>[2x]HHHHHHSSGLVPRGSHMQETQAVEAGEKTVEQFVQALNKGDYNKAAGMASKKAANKSALSEKEILEKYQNIYGAADVKGLEISNLKVDKKDDSTYSFSYKAKMNTSLGELKDLSYKGTLDRNDGKTTINWQPNLVFPEMEGNDKVSLTTQEATRGNILDRNGEPLATTGKLKQLGVVPSKLGDGDEKTANIKAIASAFDLTEDAINQAISQSWVQPDYFVPLKIIDGATPELPAGATIQEVDGRYYPLGEAAAQLIGYVGDITAEDIDKNPELSSNGKIGRSGLEMAFDKDLRGTTGGKLSITDTDGVEKKVLIEHEVQNGKDIKLTIDAKAQKTAFDSLGGKAGSTVATTPKTGDLLALASSPSYDPNKMTNGISQEDYKAYEENPEQPFI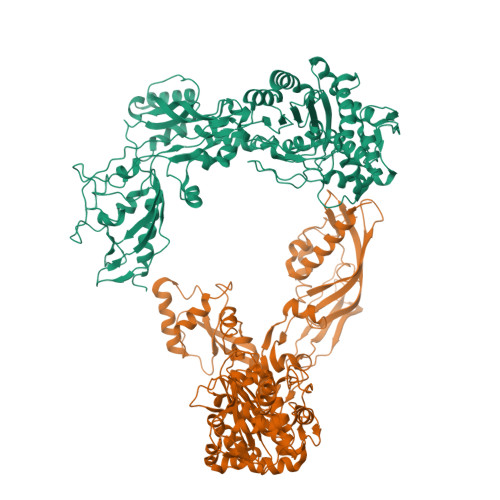SRFATGYAPGSTFKMITAAIGLDNGTIDPNEVLTINGLKWQKDSSWGSYQVTRVSDVSQVDLKTALIYSDNIYMAQETLKMGEKNFRAGLDKFIFGEDLDLPISMNPAQISNEESFNSDILLADTGYGQGELLINPIQQAAMYSVFANNGTLVYPKLIADKETKDKKNVIGETAVQTIVPDLREVVQDVNGTAHSLSALGIPLAAKTGTAEIKEKQDEKGKENSFLFAFNPDNQEYMMVSMLENKEDDDSATKRAPELLQYLNQNYQ> XPLVVAASIIAILHLILWILDR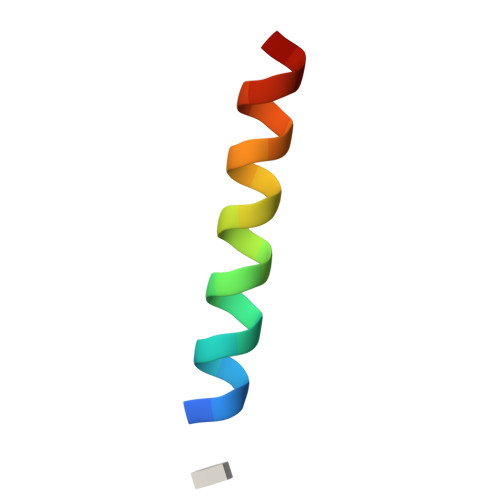LX(betaS)-Nalpha-{4-[4-(4-aminophenyl)buta-1,3-diyn-1-yl]benzoyl}-N,beta-dihydroxy-L-tyrosinamide 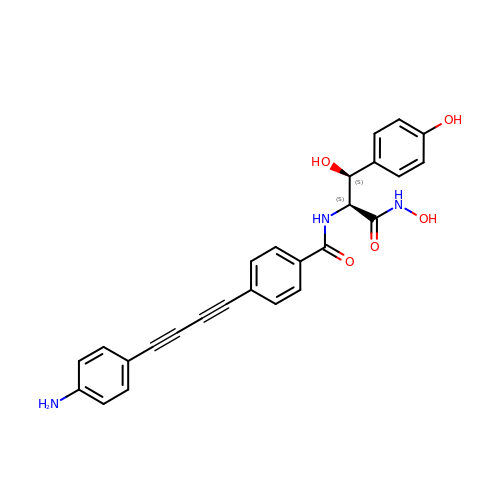| C26 H21 N3 O5 | WYPQPFTULGRIPE-ZEQRLZLVSA-N> MGNILPSWLRVGMNIAMLGMIHSDIRLITV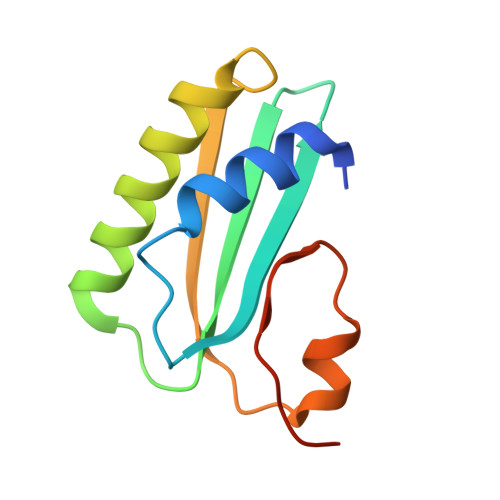DYEERRRFLKIKNYLSREAITEDHEDMEYLITELWSMCGEYFDEADFECIYSNHSSMELNQINGAVFRRKELISQALE>NLKVEFYNSN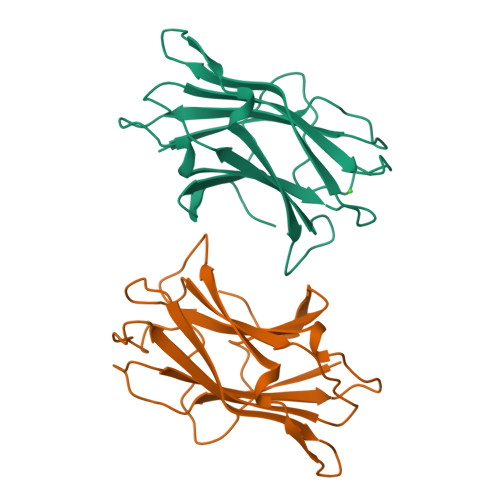PSDTTNSINPQFKVTNTGSSAIDLSKLTLRYYYTVDGQKDQTFWCDHAAIIGSNGSYNGITSNVKGTFVKMSSSTNNADTYLEISFTGGTLEPGAHVQIQGRFAKNDWSNYTQSNDYSFKSASQFVEWDQVTAYLNGVLVWGKEP[2x]>[8x]MTDQATPNLPSRDFDSTAAFYERLGFGIVFRDAGWMILQRGDLMLEFFAHPGLDPLASWFSCCLRLDDLAEFYRQCKSVGIQETSSG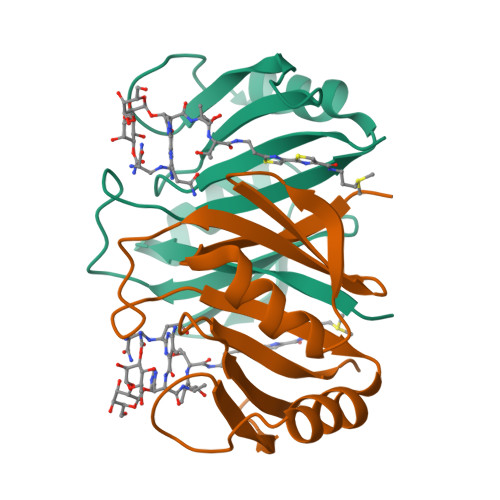YPRIHAPELQEWGGTMAALVDPDGTLLRLIQNELLAGIS>MKFPHDFLFGAASASYQVEGAWNEDGKGVTNWDEFSKIPGKTYNGTNGDIAVDHYHRYKEDVRLMAEMGLESYRFSISWARILPTGDGKVNEKGIEFYNNLIDECLKYGIVPFVTLYHWDLPLPLEKDGGWTNKRTAEAFVKYAETCFKAFGDRVKHWITFNETVMFCGLGYLKGAHPPGIQNDVPKYFQATHYVFYAHAKTVAVYKQLKQYGEIGITHVFLPAYSVDDQKENIQAANHANEYETYWYYDPILKGE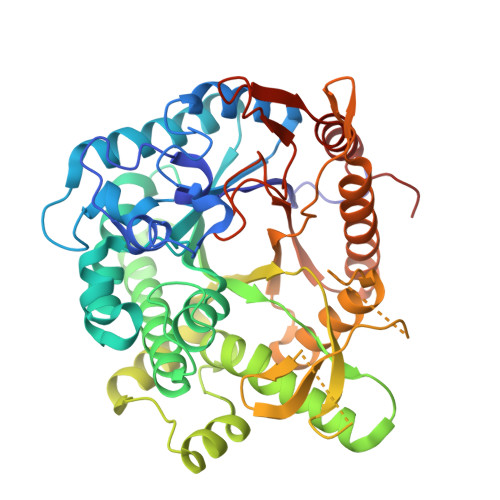YPSYVVQQLKEKGWTPNWTVEELEIIKQNAEENDFIGLNYYQPIRVERYDMDIKSEEHSRENSTLAPGNPSFDGFYRTVKMDDKTYTKWGWEISPEGFLEGLHMLKARYGDIKMYVTENGLGDEDPIIDGEIVDVPRIKFIEAHLKVMKRAIEEGINLKGYYAWSVIDLLSWLNGYKKQYGFIFVDHNDNLKRKKKLSFHWYKRVVETRGEELHHHHHH[2x]> MIKAILIFNNHGKPRLSKFYQPYSEDTQQQIIRETFHLVSKRDENVCNFLEGGLLIGGSDNKLIYR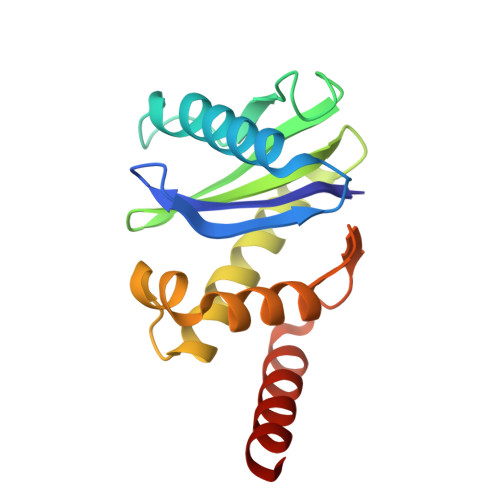HYATLYFVFCVDSSESELGILDLIQVFVETLDKCFENVCELDLIFHVDKVHNILAEMVMGGMVLETNMNEIVTQIDAQNKLEKSE> MHGRLKVKTSEEQAEAKRLEREQKLKLYQSATQAVFQKRQAGELDESVLELTSQILGANPDFATLWNCRREVLQHLETEKSPEESA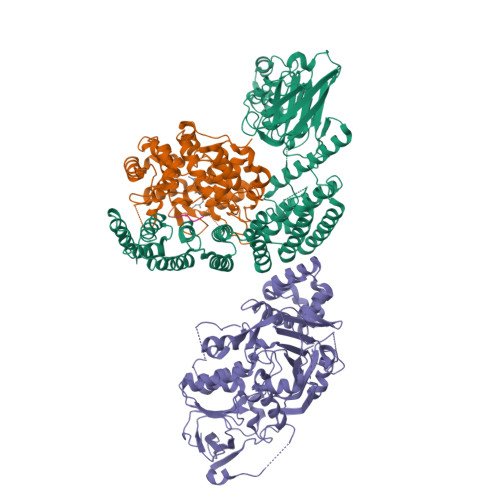ALVKAELGFLESCLRVNPKSYGTWHHRCWLLSRLPEPNWARELELCARFLEADERNFHCWDYRRFVAAQAAVAPAEELAFTDSLITRNFSNYSSWHYRSCLLPQLHPQPDSGPQGRLPENVLLKELELVQNAFFTDPNDQSAWFYHRWLLGRAEPHDVLCCVHVSREEACLSVCFSRPLTVGSRMGTLLLMVDEAPLSVEWRTPDGRNRPSHVWLCDLPAASLNDQLPQHTFRVIWTGSDSQKECVLLKDRPECWCRDSATDEQLFRCELSVEKSTVLQSELESCKELQELEPENKWCLLTIILLMRALDPLLYEKETLQYFSTLKAVDPMRAAYLDDLRSKFLLENSVLKMEYADVRVLHLAHKDLTVLCHLEQLLLVTHLDLSHNRLRALPPALAALRCLEVLQASDNALENVDGVANLPRLQELLLCNNRLQQSAAIQPLVSCPRLVLLNLQGNSLCQEEGIQERLAEMLPSVSSILT;> MGTQQKDVTIKSDAPDTLLLEKHADYIASYGSKKDDYEYCMSEYLRMSGVYWGLTVMDLMGQLHRMNKEEILVFIKSCQHECGGVSASIGHDPHLLYTLSAVQILTLYDSIHVINVDKVVAYVQSLQKEDGSFAGDIWGEIDTRFSFCAVATLALLGKLDAINVEKAIEFVLSCMNFDGGFGCRPGSESHAGQIYCCTGFLAITSQLHQVNSDLLGWWLCERQLPSGGLNGRPEKLPDVCYSWWVLASLKIIGRLHWIDREKLRSFILACQDEETGGFADRPGDMVDPFHTLFGIAGLSLLGEEQIKPVSPVFCMPEEVLQRVNVQPELVS;> AAAA;> MADNLPSDFDVIVIGTGLPESIIAAACSRSGQRVLHVDSRSYYGGNWASFSFSGLLSWLKEYQENNDVVTENSMWQEQILENEEAIPLSSKDKTIQHVEVFCYASQDLHKDVEEAGALQKNHASVTSAQSAEAAEAAETSCLPTAVEPLSMGSCEIPAEQSQCPGPESSPEVNDAEATGKKENSDAKSSTEEPSENVPKVQDNTETPKKNRITYSQIIKEGRRFNIDLVSKLLYSRGLLIDLLIKSNVSRYAEFKNITRILAFREGTVEQVPCSRADVFNSKQLTMVEKRMLMKFLTFCVEYEEHPDEYRAYEGTTFSEYLKTQKLTPNLQYFVLHSIAMTSETTSCTVDGLKATKKFLQCLGRYGNTPFLFPLYGQGELPQCFCRMCAVFGGIYCLRHSVQCLVVDKESRKCKAVIDQFGQRIISKHFIIEDSYLSENTCSRVQYRQISRAVLITDGSVLKTDADQQVSILTVPAEEPGSFAVRVIELCSSTMTCMKGTYLVHLTCMSSKTAREDLERVVQKLFTPYTEIEAENEQVEKPRLLWALYFNMRDSSDISRDCYNDLPSNVYVCSGPDSGLGNDNAVKQAETLFQQICPNEDFCPAPPNPEDIVLDGDSSQQEVPESSVTPETNSETPKESTVLGNPEEPSE> DPDQFRAIIESPEGAGHVGYQYRRNTGSTMRMVSDVLDERVSLWDFHCDPSGNVIQPGPNVDSRQYLQAAIDYVSSNGGGTITIPAGYTWYLGSYGVGGIAGHSGIIQLRSNVNLNIEGRIHLSPFFDLKPFQVFVGFDNGDPASSGNLENCHIYGHGVVDFGGYEFGASSQLRNGVAFGRSYNCSVTGITFQNGDVTWAITLGWNGYGSNCYVRKCRFINLVNSSVNADHSTVYVNCPYSGVESCYFSMSSSFARNIACSVELHQHDTFYRGSTVNGYCRGAYVVMHAAEAAGAGSYAYNMQVENNIAVIYGQFVILGSDVTATVSGHLNDVIVSGNIVSIGERAAFSAPFGAFIDIGPDNSGASNVQDIQRVLVTGNSFYAPANITDSAAITLRANLNGCTFIANNFDCRYMVYNAPGTTSPVVQNLVWDKSNVIGGTHANQRAGQNLFDMQFAS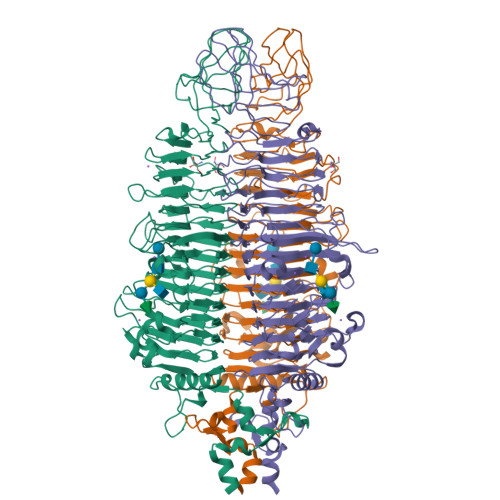VVNSTIEVQLSCEDLSMFSCILFPASCQLSYSKITVDSAWTKSMSNTAVFEGNQQAGANVYVSYPATVNLTSYNTQGAVPFFSTDTNYAWVTSAYSLSINENLDFSPPATYTNKANGQLVGVGYNEIGGVRSVSVRLMLQRQV>GGGTTGGGTTGGGTTGGG[2x]

G-quadruplex (GQ) DNA is a well-studied non-canonical DNA structure formed by the π-π stacking of G-quartets. Here, we investigate the interaction of T1 with N-methyl mesoporphyrin IX (NMM), a water-soluble porphyrin with a distinctive central methyl group. Driven by this gap in knowledge, we determined crystal structures of T1-NMM and T7-NMM to 2.39 and 2.34 Å, respectively, as well as characterized stoichiometry, strength, and thermodynamic parameters of the T1-NMM interaction.

In solution, T1 exists mostly as a dimer of parallel GQs. The T1-NMM crystal structure was solved in the R 3 2 space group to 2.39 Å. In both cases, the asymmetric unit contains two DNA chains, each of which binds one NMM molecule. Meanwhile, for T1-NMM, there may be stacking between T4 in chain A and T14 in chain B, but the electron density for T14 is poor and its base was not built. *NMM molecule bound to chain B was modeled in two different orientation each at 0.5 occupancy; one potassium ion rests on the special position at the dimer interface and was modeled at 0.5 occupancy in each monomer. According to PAGE, T1-NMM exists as a mixture of monomer and dimer regardless of concentration. Meanwhile, T7 is a monomer alone as well as in complex with NMM at both high and low concentrations. This data suggests that the T1 dimer observed in the crystal structure could exist under physiological conditions. In summary, our extensive binding studies demonstrate that NMM binds T1 with 1:1 stoichiometry and an extremely tight binding constant of 30–50 μM-1. The binding of NMM to T1 is characterized by an unprecedentedly high binding affinity of 30–50 μM-1, the strongest reported for any GQ-NMM complex. The impressive binding of NMM to T1 is also accompanied by 20 °C of stabilization at 2 eq. of NMM, the highest observed for any GQ.>GPGSMANDYLFTSESVSEGHPDKVADQISDAILDAILAQDKYSRVAAETLCNTGLVVLAGEITTTANIDYIQIARDTIKRIGYDNTDYGIDYRGCAVLVAYDKQSPDIAQGVDRAHDNNLDQGAGDQGLMFGYACDETPELMPLPIHLSHRLVERQANLRRDG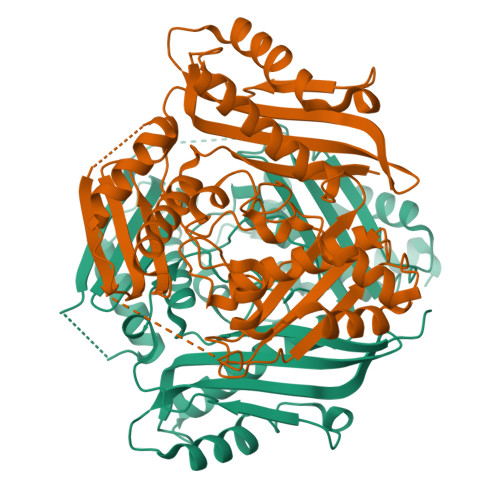RLPWLRPDAKSQVTVRYVDGKPHSIDTVVLSTQHAPEIDLPALREAVIEEVIKPTLPADLIKGDIKFLVNPTGRFVIGGPQGDCGLTGRKIIVDTYGGAAPHGGGAFSGKDPSKVDRSAAYAGRYVAKNIVAAGLASRALIQVSYAIGVAEPTSVMVNTFGTGRVSDETITKLVREHFDLRPKGIIQMLDLLRPIYEKTAAYGHFGREEPEFSWEAADKALALAEAAGVEPAVQVA[4x]> DSQRSTLVHWFRKGLRLHDNPALSHIFTAANAAPGRYFVRPIFILDPGILDWMQVGANRWRFLQQTLEDLDNQLRKLNSRLFVVRGKPAEVFPRIFKSWRVEMLTFETDIEPYSVTRDAAVQKLAKAEGVRVETHCSHTIYNPELVIAKNLGKAPITYQKFLGIVEQLKVPKVLGVPEKLKNMPTPPKDEVEQKDSAAYDCPTMKQLVKRPEELGPNKFPGGETEALRRMEESLKDEIWVARFEKPNTAPNSLEPSTTVLSPYLKFGCLSARLFNQKLKEIIKRQPKHSQPP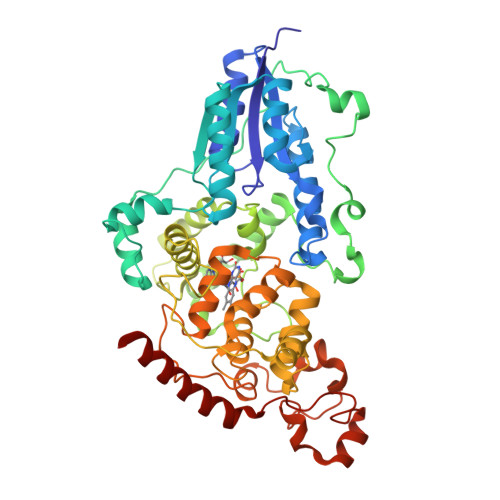VSLIGQLMWREFYYTVAAAEPNFDRMLGNVYCMQIPWQEHPDHLEAWTHGRTGYPFIDAIMRQLRQEGWIHHLARHAVACFLTRGDLWISWEEGQRVFEQLLLDQDWALNAGNWMWLSASAFFHQYFRVYSPVAFGKKTDPQGHYIRKYVPELSKYPAGCIYEPWKASLVDQRAYGCVLGTDYPHRIVKHEVVHKENIKRMGAAYKVNRE>MSENPLLERARRFLSALRHCQVLGLTVEAADEKGLTLRLPYSQAIIGNPESGVVHGGAITTLMDTTCG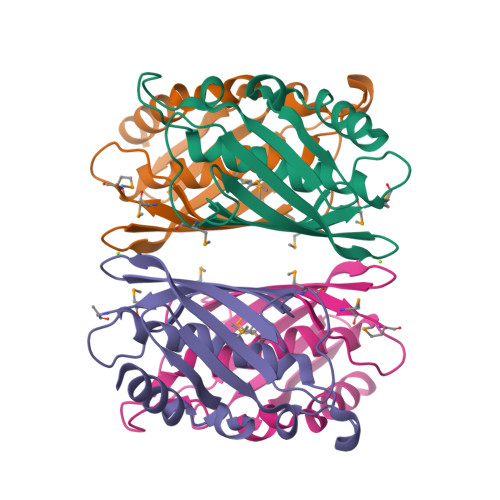ISTVCVLPDFEICPTLDLRIDYMHPAEPHKDVYGFAECYRVTPNVIFTRGFAYQDDPGQPIAHVVGAFMRMGLEHHHHHH[4x]>ACCGACGTCGGT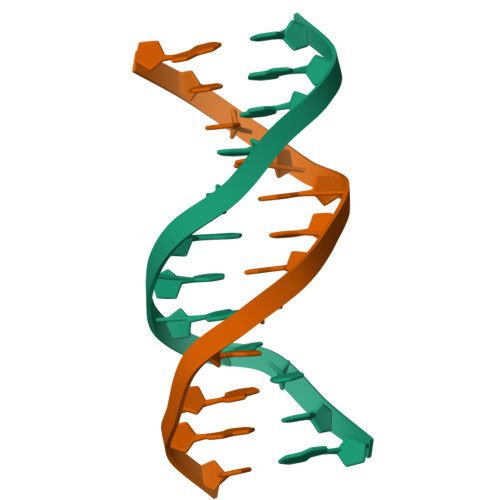[6x]> ISGGDAIYSSTGRCSLGFNVRSGSTYYFLTAGHCTDGATTWW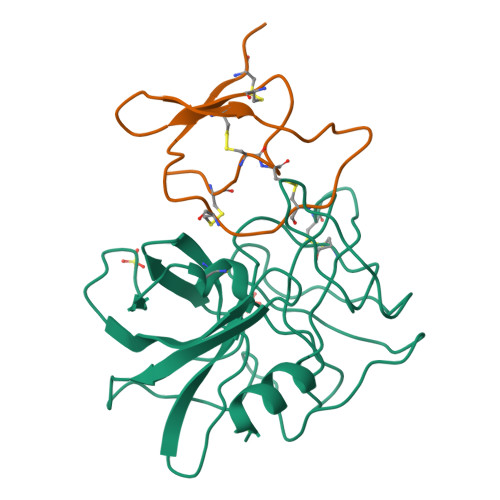ANSARTTVLGTTSGSSFPNNDYGIVRYTNTTIPKDGTVGGQDITSAANATVGMAVTRRGSTTGTHSGSVTALNATVNYGGGDVVYGMIRTNVCAEPGDSGGPLYSGTRAIGLTSGGSGNCSSGGTTFFQPVTEALVAYGVSVY;> PICTNCCAGYKGCNYYSANGAFICEGQSDPKKPKACPLNCDPHIAYSKCPR> AHHHHHHMQGSVTEFLKPRLVDIEQVSSTHAKVTLEPLERGFGHTLGNALRRILLSSMPGCAVTEVEIDGVLHEYSTKEGVQEDILEILLNLKGLAVRVQGKDEVILTLNKSGIGPVTAADITHDGDVEIVKPQHVICHLTDENASISMRIKVQRGRGYVP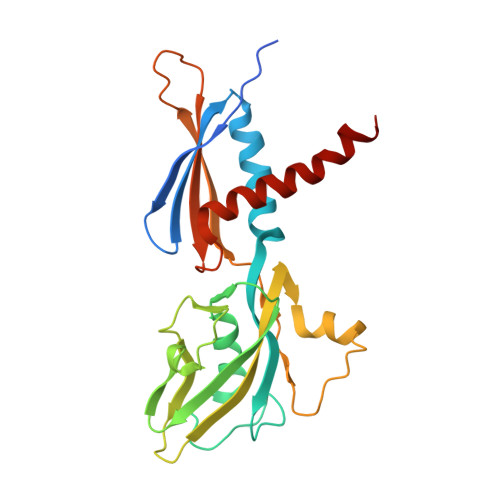ASTRIHSEEDERPIGRLLVDACYSPVERIAYNVEAARVEQRTDLDKLVIEMETNGTIDPEEAIRRAATILAEQLEAFVDLR>[2x]MSITSDEVNFLVYRYL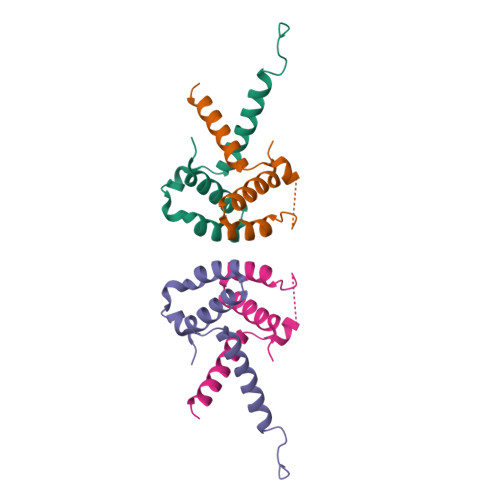QESGFSHSAFTFGIESHISQSNINGTLVPPAALISILQKGLQYVEAEISINEDGTVFDGRPIESLSLIDAVMPD>[2x]QAQITGRPEWIWLALGTALMGLGTLYFLVKGMGVSDPDAKKFYAITTLVAAIAFTMYLSMLLGYGLTMVPFGGEQNPIYWARYADWL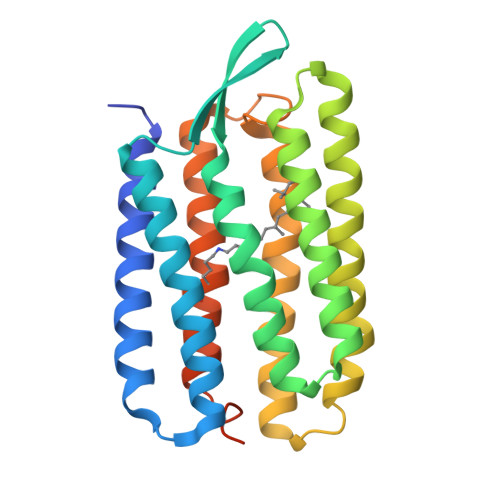FTTPLLLLDLALLVDADQGTILALVGADGIMIGTGLVGALTKVYSYRFVWWAISTAAMLYILYVLFFGFTSKAESMRPEVASTFKVLRNVTVVLWSAYPVVWLIGSEGAGIVPLNIETLLFMVLDVSAKVGFGLILLRSRAIFGEAEAPEPSAGDGAAATSD> MSQSNRELVVDFLSYKLSQKGYSWSQMAAVKQA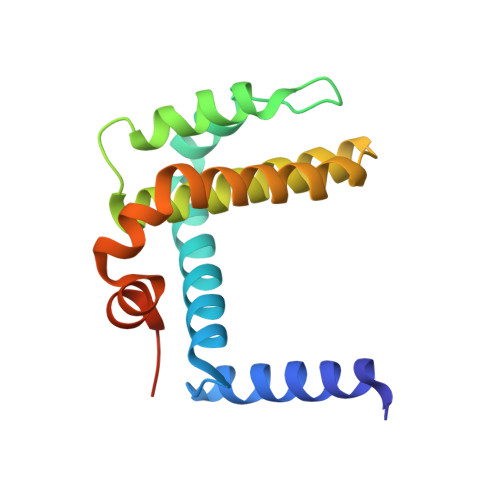LREAGDEFELRYRRAFSDLTSQLHITPGTAYQSFEQVVNELFRDGVNWGRIVAFFSFGGALCVESVDKEMQVLVSRIAAWMATYLNDHLEPWIQENGGWDTFVELYGNNAAAESRKGQER> MPQQLSPINIETKKAISNARLKPLDIHYNESKPTTIQNTGKLVRINFKGGYISGGFLPNEYVLSSLHIYWGKEDDYGSNHLIDVYK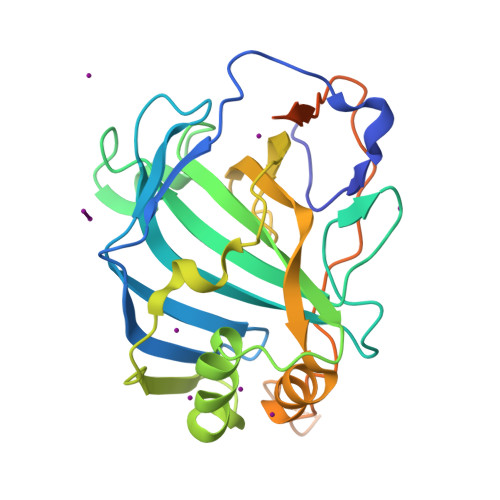YSGEINLVHWNKKKYSSYEEAKKHDDGLIIISIFLQVLDHKNVYFQKIVNQLDSIRSANTSAPFDSVFYLDNLLPSKLDYFTYLGTTINHSADAVWIIFPTPINIHSDQLSKFRTLLSLSNHEGKPHYITENYRNPYKLNDDTEVYYSGEIIRAATTSPARENYFMRWLSDLRETLEHHHHHH>MATPHINAEMGDFADVVLMPGDPLRAKYIAETFLEDAREVNNVRGMLGFTGTYKGRKISVMGHGMGIPSCSIYTKELITDFGVKKIIRVGSCGAVLPHVKLRDVVIGMGACTDSKVNRIRFKDHDFAAIADFDMVRNAVDAAKALGIDARVGNLFSADLFYSPDGEMFDVMEKYGILGVEMEAAGIYGVAAEFGAKALTICTVSNHIRTHEQTTAAERQTTFNDMIKIALESVLLG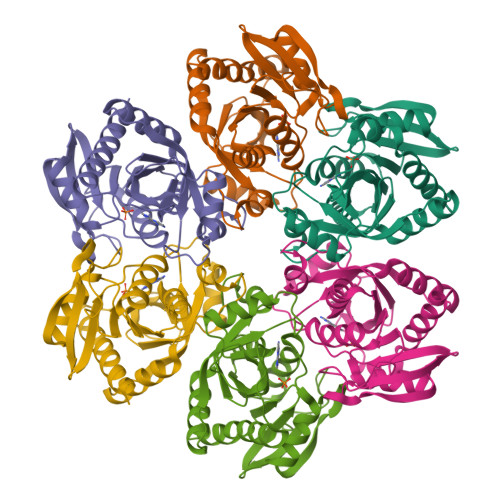DKE[3x]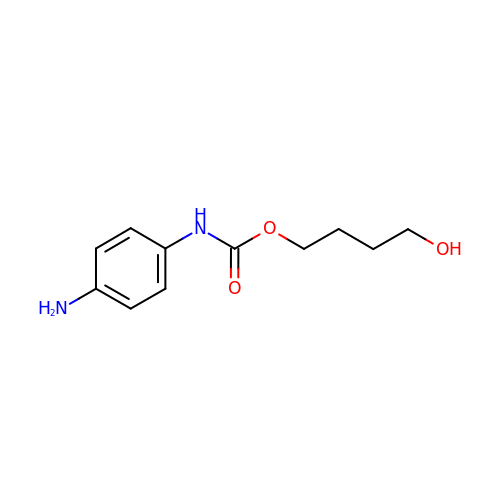4-oxidanylbutyl ~{N}-(4-aminophenyl)carbamate | C11 H16 N2 O3 | UEFKPOWGEZOFJI-UHFFFAOYSA-N> ERTINLYPLTNYTFGTKEPLYEKDSSVAARFQRMREEFDKIGMRRTVEGVLIVHEHRLPHVLLLQLGTTFFKLPGGELNPGEDEVEGL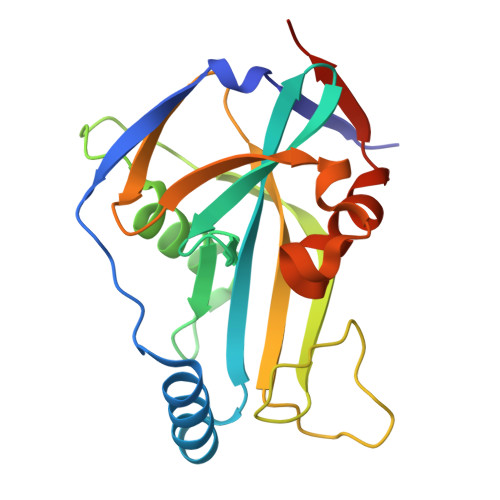KRLMTEILGRQDGVLQDWVIDDCIGNWWRPNFEPPQYPYIPAHITKPKEHKKLFLVQLQEKALFAVPKNYKLVAAPLFELYDNAPGYGPIISSLPQLLSRFNFIYNLEHHHHHH> VEGRFQLVAPYEPQGDQPQAIAKLVDGLRRGVKHQTLLGATGTGKTFTISNVIAQVNKPTLVIAHNKTLAGQLYSELKEFFPHNAVEYFVSYYDYYQPEAYVPQTDTYIEKDAKINDEIDKLRHSATSALFERRDVIIVASVSCIYGLGSPEEYRELVVSLRVGMEIERNALLRRLVDIQYDRNDIDFRGTFRVRGDVVEIFPASRDEHCIRVEFFGDEIERIRAEVDALTGKVLGEREHVAIFPASHFVTREEKMRLAIQNIEQELEERLAELRAQGKLLEAQRLEQRTRYDLEMMREMGFCSGIENYSRHLALRPPGSTPYTLLDYFPDDFLIIVDESHVTLPQLRGMYNGDRARKQVLVDHGFRLPSALDNRPLTFEEFEQKINQIIYVSATPGPYELEHSPGVVEQIIRPTGLLDPTIDVRPTKGQIDDLIGEIRERVERNERTLVT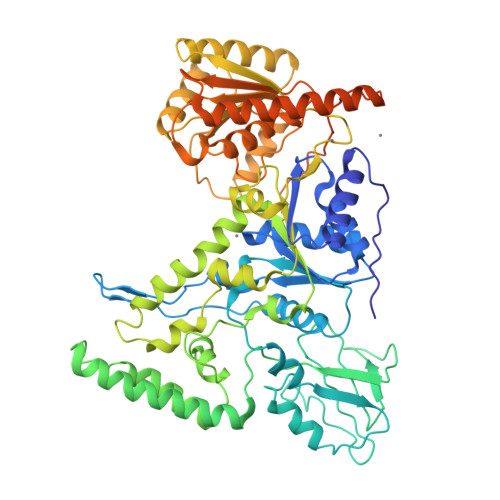TLTKKMAEDLTDYLKEAGIKVAYLHSEIKTLERIEIIRDLRLGKYDVLVGINLLREGLDIPEVSLVAILDADKEGFLRSERSLIQTIGRAARNANGHVIMYADTITKSMEIAIQETKRRRAIQEEYNRKHGIVPRTVKKEIRDVIRATYAAEETEMYEAKPAAAMTKQEREELIRTLEAEMKEAAKALDFERAAQLRDIIFELKAEG>MWRYPRNADQTFWAFRTCQRQSEGAKSLREWYRWNLPNDEDTHCYVKCVWLHLGLYNEQNKSLRVDRIMEQFNSRSVAIPGGINTISGPTDGTCKDIYDKTINFFNNNVNDLRTAFYGIKKLSDEWFTQNSNTKPKGTKISDFCNAENREKGGADCQHACSAYYYRLVDEDNEPIHFRNLNILGITDEQFASCVKASKNKQGCKVADTMYNCVEKHNSQALKILDNQSPTY[2x]

Despite the ‘rule of thumb’ that blood feeders from independent evolutionary lineages utilize different protein families for various salivary functions, the saliva of sand flies contains apparent homologs of the two-domain long-form D7 proteins of mosquitoes. In this study we demonstrate, using binding studies and bioassays, that the sand fly long-form D7s do in fact bind both cysteinyl leukotrienes and thromboxanes, and thereby serve as anti-inflammatory and anti-hemostatic agents in both sandflies and mosquitoes. In this study we show that the long-form D7 proteins from sand flies are functionally like their counterparts in mosquito saliva and share a conserved structure. Consistent with these structural observations, the sand fly proteins were found to perform the same anti-inflammatory and anti-platelet functions as their mosquito counterparts through the binding of cysteinyl leukotrienes and TXA2 in the N-terminal domain, but do not bind biogenic amines, as this function is performed by the yellow proteins.

The structure of ABI15936 was determined using single anomalous diffraction methods with a selenomethionine-substituted variant protein prepared in E. coli. An initial model containing two protein monomers was built using the experimental electron density map and then positioned into a wild-type data set by molecular replacement. The model was then completed by iterative cycles of rebuilding and refinement. As suggested by sequence comparisons, the protein is made up of two linked odorant binding protein (OBP) domains with a well-ordered domain interface fixing their relative orientations. Although ABI15936 was crystallized in the absence of any potential natural ligands, electron density was observed indicative of a non-protein molecule occupying the N-terminal domain binding site. This was determined after refinement of the protein complex to be the detergent Triton X-100, which was retained through the steps of protein purification. The binding pocket of ABI15936 is much like that of the mosquito long-form D7 proteins, with numerous residues important for ligand binding being conserved. In the structure of ABI15936, Tyr 44 is oriented identically to the homologous residue Tyr 52 in AnStD7L1 and can be assumed to play the same role in binding. The C-terminal domain of ABI15936 shows a clear structural relationship to mosquito long-form D7s but the protein does not contain the interior binding pocket known to accommodate biogenic amine ligands in the long-form D7 AeD7 from Ae. aegypti and the short-form D7 protein D7r4 from An. gambiae. Comparison of ABI15936 with AeD7 shows that the region connecting helices α9 and α10 is truncated relative to AeD7, eliminating the equivalent of α-helix B2 of AeD7 that makes up one side of the ligand binding pocket.> MAIEKGEAFARRDIY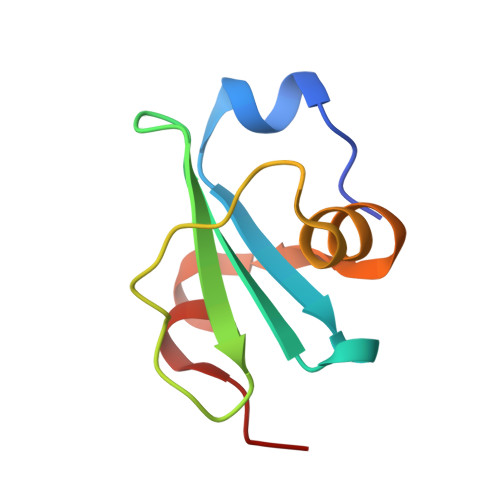IDYDFEDVTYRWDHRQGTIHVRFYGEAESPEPVEHDNRLFNDALRFGREITREEYETGFPKG>[4x]MKKENQTQEIEERYQALFSNAAAVKALTQVVANSLGPKGLDAMLVDRFGEVVVTNDGVTILTLMDAQHPAARMVVNMARAQEREVGDGTTTAAVLAGALVSEGVNQILKGVPVSKVLAGMNRALNHALFLIRKNAIKVGSITDDRLLAAAKIAGRGDERVAAILRDAAAMLEDKLQDPGFKLADLVLAKVGADTTLIPGVVINKSPLWEEGSQKLQEVRLLVLDDGLYPEEVEEEALASEAGFEQYLKNQKIFQENLKKLKELGVKLILLTRGISDIAEEFCYENEIMVITRIT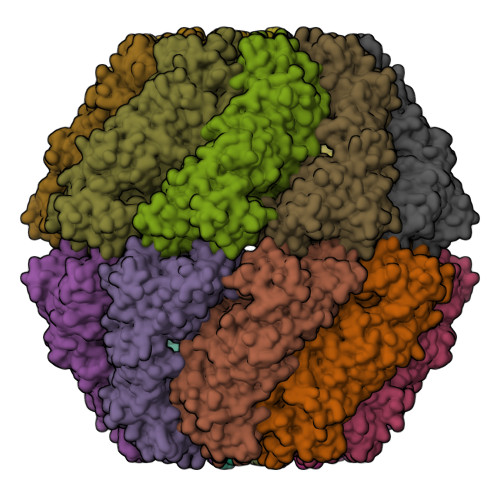QKELKRVLEFTGARAAKRTSLNKPVEELQKMLGYARTCFYDSRLDFTIIEGGAGKATATVLIGAATDEVVDEQERIAKDAAGSFAAAYRSGVLPGGGAFFLYLSREVESLKNRLPGMESYGVMAFSEALKVPFRVMAENAGFNGLEKLGDLMTLQVQKNNYALGLDFETGEFIDMIAGGVVDPAEVVYQAVKNASEVAISLLKINTIIKMKDYEVLKEGEQEDGGKR>[12x]MRLCDRDIEAWLDEGRLSINPRPPVERINGATVDVRLGNKFRTFRGHTAAFIDLSGPKDEVSAALDRVMSDEI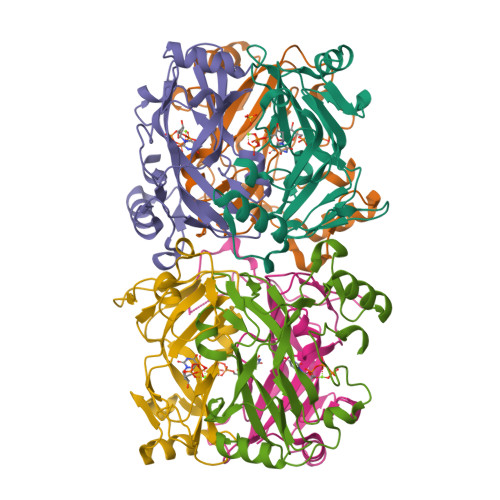VLDEGEAFYLHPGELALAVTLESVTLPADLVGWLDGRSSLARLGLMVHVTAHRIDPGWSGCIVLDFYNSGKLPLALRPGMLIGALSFEPLSGPAVRPYNRREDAKYRNQQGAVASRIDKD>MNAHAPSVAPASATVDASLEKLERKPVLVASRDLPALAVIGRDDLSVELLRTAPVGSYDRPEALLGKRVWVAVPAGSILSAATLEPGGPLARTIRPDERAMAIAVDEVVGGGGFVLPGDYVDVMLFVRDERDGESTPLAQLVLPGVRVLTYGERIAVGSDGQDRSNQEKDPRPPRTAVLAVPEDGVARLMLASQAGSLRLAIRSKDEELYRREQEGALLQAS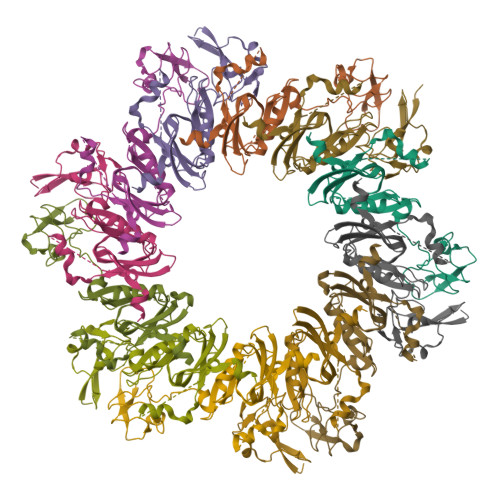LGAPSAALSLDQLLERRKPTAPSVRSAAPRVPVANGVTVYRGSAMTHEAPLEHHHHHH[12x]>[2x]MSNKCDVVVVGGGISGMAAAKLLHDSGLNVVVLEARDRVGGRTYTLRNQKVKYVDLGGSYVGPTQNRILRLAKELGLETYKVNEVERLIHHVKGKSYPFRGPFPPVWN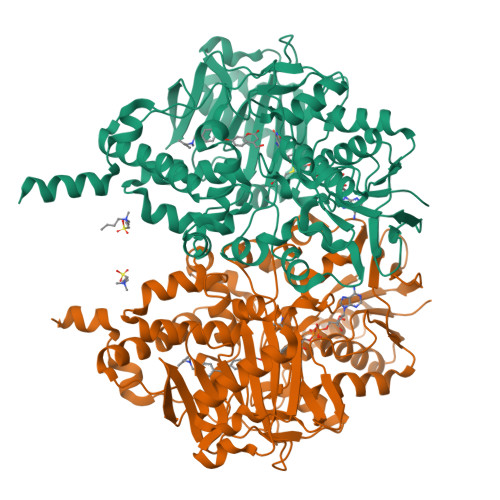PITYLDHNNFWRTMDDMGREIPSDAPWKAPLAEEWDNMTMKELLDKLCWTESAKQLATLFVNLCVTAETHEVSALWFLWYVKQCGGTTRIISTTNGGQERKFVGGSGQVSERIMDLLGDRVKLERPVIYIDQTRENVLVETLNHEMYEAKYVISAIPPTLGMKIHFNPPLPMMRNQMITRVPLGSVIKCIVYYKEPFWRKKDYCGTMIIDGEEAPVAYTLDDTKPEGNYAAIMGFILAHKARKLARLTKEERLKKLCELYAKVLGSLEALEPVHYEEKNWCEEQYSGGCYTTYFPPGILTQYGRVLRQPVDRIYFAGTETATHWSGYMEGAVEAGERAAREILHAMGKIPEDEIWQSEPESVDVPAQPITTTFLERHLPSVPGLLRLIGLTTIFSATALGFLAHKRGLLVRV> QDDSTPDSLFAGLVGEYYGTNSQLNNISDFRALVDSKEADATFEAANISYGRGSSDVAKGTHLQEFLGSDASTLSTDPGDNTDGGIYLQGYVYLEAGTYNFKVTADDGYEIT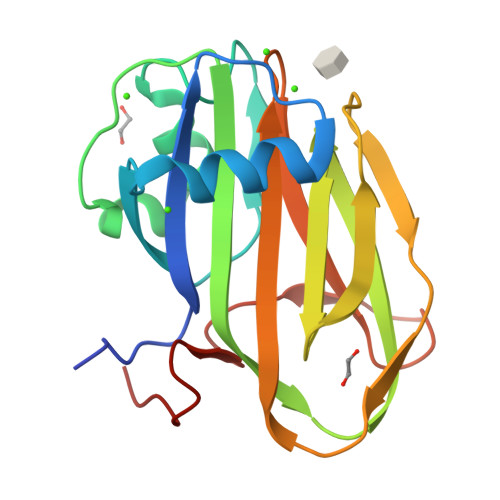INGNPVATVDNNQSVYTVTHASFTISESGYQAIDMIWWDQGGDYVFQPTLSADGGSTYFVLDSAILSSTGETPYTT Human SMG1 is one of the largest PIKK family members (~410 kDa) and plays a crucial role in nonsense-mediated mRNA decay (NMD), a conserved pathway that regulates mRNA stability in the cytoplasm of eukaryotic cells. In metazoans, SMG1 forms a stable complex with two additional proteins, SMG8 and SMG9, and specifically phosphorylates the RNA helicase UPF1. SMG1 phosphorylates UPF1 specifically at Ser/Thr - Gln (SQ) motifs present in the unstructured N- and C-terminal regions that flank the helicase core. Briefly, SMG1 consists of an N-terminal solenoid 'arch' and a compact C-terminal 'head' region.

For structure determination, we incubated SMG1-8-9 with UPF1-LSQ and AMPPNP, a non-hydrolyzable ATP analogue, and subjected the sample to cryo-EM single particle analysis. The final reconstruction reached an overall resolution of 2.9 Å (Figure 1—figure supplements 2 and 3), and allowed us to further complete and refine the published model for SMG1-8-9 (Gat et al., 2019). Importantly, compared to the previously published apo-SMG1-8-9 structure, the current reconstruction revealed extra density in the kinase active site accounting for both AMPPNP and UPF1-LSQ. The active site of SMG1 shows excellent density for residues 1075–1081 of UPF1-LSQ. The hydroxyl group of Ser1078, the phospho-acceptor residue in UPF1-LSQ, is positioned by residues of the catalytic loop, in particular Asp2335 and His2337. In our structure, the glutamine at position +1 of UPF1-LSQ reaches into a hydrophobic cage formed by the SMG1 activation segment and FATC domain. In particular, UPF1 Gln1079 stacks against Tyr3654 and Leu2365 and forms hydrogen bonds with the backbone of Val2367. In our model, the Leu residue at position −1 in the substrate forms a C-H⋅⋅⋅π-interaction with SMG1 Phe2215 and is further stabilized by hydrophobic interactions with SMG1 Pro2249 and Gly3656. The local resolution of around 3 Å allowed us to model SMG9-bound ATP in the reconstructed density, revealing the molecular basis for how the adenosine nucleotide is recognized by this unusual G-fold domain. In this manuscript, we report the first structure of a substrate-bound PIKK active site, thereby revealing the basis for phosphorylation site selection by SMG1 and other PIKK family members.

> XXXXXXXXXXXXXXXXXXXXXXXXXXXXXXXXXXXXXXXXXXXXXXXXXXXXXXXXXXXXXXXXXXXXXALETVGEKKAFSSVMQLVMTSLQSILENVDTPELLCKCVKCILLVARCYPHIFSTNFRDTVDILVGWHIDHTQKPSLTQQVSGWLQSLEPFWVADLAFSTTLLGQFLEDMEAYAEDLSHVASGESVDEDVPPPSVSLPKLAALLRVFSTVVRSIGERFSPIRGPPITEAYVTDVLYRVMRCVTAANQVFFSEAVLTAANECVGVLLGSLDPSMTIHCDMVITYGLDQLENCQTCGTDYIISVLNLLTLIVEQINTKLPSSFVEKLFIPSSKLLFLRYHKEKEVVAVAHAVYQAVLSLKNIPVLETAYKLILGEMTCALNNLLHSLQLPEACSEIKHEAFKNHVFNVDNAKFVVIFDLSALTTIGNAKNSLIGMWALSPTVFALLSKNLMIVHSDLAVHFPAIQYAVLYTLYSHCTRHDHFISSSLSSSSPSLFDGAVISTVTTATKKHFSIILNLLGILLKKDNLNQDTRKLLMTWALEAAVLMRKSETYAPLFSLPSFHKFCKGLLANTLVEDVNICLQACSSLHALSSSLPDDLLQRCVDVCRVQLVHSGTRIRQAFGKLLKSIPLDVVLSNNKHTEIQEISLALRSHMSKAPSNTFHPQDFSDVISFILYGNSHRTGKDNWLERLFYSCQRLDKRDQSTIPRNLLKTDAVLWQWAIWEAAQFTVLSKLRTPLGRAQDTFQTIEGIIRSLAAHTLNPDQDVSQWTTADNDEGHGNNQLRLVLLLQYLENLEKLMYNAYEGCANALTSPPKVIRTFFYTNRQTCQDWLTRIRLSIMRVGLLAGQPAVTVRHGFDLLTEMKTTSLSQGNELEVTIMMVVEALCELHCPEAIQGIAVWSSSIVGKNLLWINSVAQQAEGRFEKASVEYQEHLCAMTGVDCCISSFDKSVLTLANAGRNSASPKHSLNGESRKTVLSKPTDSSPEVINYLGNKACECYISIADWAAVQEWQNSIHDLKKSTSSTSLNLKADFNYIKSLSSFESGKFVECTEQLELLPGENINLLAGGSKEKIDMKKLLPNMLSPDPRELQKSIEVQLLRSSVCLATALNPIEQDQKWQSITENVVKYLKQTSRIAIGPLRLSTLTVSQSLPVLSTLQLYCSSALENTVSNRLSTEDCLIPLFSEALRSCKQHDVRPWMQALRYTMYQNQLLEKIKEQTVPIRSHLMELGLTAAKFARKRGNVSLATRLLAQCSEVQLGKTTTAQDLVQHFKKLSTQGQVDEKWGPELDIEKTKLLYTAGQSTHAMEMLSSCAISFCKSVKAEYAVAKSILTLAKWIQAEWKEISGQLKQVYRAQHQQNFTGLSTLSKNILTLIELPSVNTMEEEYPRIESESTVHIGVGEPDFILGQLYHLSSVQAPEVAKSWAALASWAYRWGRKVVDNASXXXXXXXXXXXXXXXXXXXXXXXXXXXXXXXXXXXXXXXXXXEGVIKVWRKVVDRIFSLYKLSCSAYFTFLKLNAGQIPLDEDDPRLHLSHRVEQSTDDMIVMATLRLLRLLVKHAGELRQYLEHGLETTPTAPWRGIIPQLFSRLNHPEVYVRQSICNLLCRVAQDSPHLILYPAIVGTISLSSESQASGNKFSTAIPTLLGNIQGEELLVSECEGGSPPASQDSNKDEPKSGLNEDQAMMQDCYSKIVDKLSSANPTMVLQVQMLVAELRRVTVLWDELWLGVLLQQHMYVLRRIQQLEDEVKRVQNNNTLRKEEKIAIMREKHTALMKPIVFALEHVRSITAAPAETPHEKWFQDNYGDAIENALEKLKXXXXXXXXXXXXXXXXYILRLEEISPWLAAMTNTEIALPGEVSARDTVTIHSVGGTITILPTKTKPKKLLFLGSDGKSYPYLFKGLEDLHLDERIMQFLSIVNTMFATINRQETPRFHARHYSVTPLGTRSGLIQWVDGATPLFGLYKRWQQREAALQAQKAQDSYQTPQNPGIVPRPSELYYSKIGPALKTVGLSLDVSRRDWPLHVMKAVLEELMEATPPNLLAKELWSSCTTPDEWWRVTQSYARSTAVMSMVGYIIGLGDRHLDNVLIDMTTGEVVHIDYNVCFEKGKSLRVPEKVPFRMTQNIETALGVTGVEGVFRLSCEQVLHIMRRGRETLLTLLEAFVYDPLVDWTAGGEAGFAGAVYGGGGQQAESKQSKREMEREITRSLFSSRVAEIKVNWFKNRDEMLVVLPKLDGSLDEYLSLQEQLTDVEKLQGKLLEEIEFLEGAEGVDHPSHTLQHRYSEHTQLQTQQRAVQEAIQVKLNEFEQWITHYQAAFNNLEATQLASLLQEISTQMDLGPPSYVPATAFLQNAGQAHLISQCEQLEGEVGALLQQRRSVLRGCLEQLHHYATVALQYPKAIFQKHRIEQWKTWMEELICNTTVERCQELYRKYEMQYAPQPPPTVCQFITATEMTLQRYAADINSRLIRQVERLKQEAVTVPVCEDQLKEIERCIKVFLHENGEEGSLSLASVIISALCTLTRRNLMMEGAASSAGEQLVDLTSRDGAWFLEELCSMSGNVTCLVQLLKQCHLVPQDLDIPNPMEASETVHLANGVYTSLQELNSNFRQIIFPEALRCLMKGEYTLESMLHELDGLIEQTTDGVPLQTLVESLQAYLRNAAMGLEEETHAHYIDVARLLHAQYGELIQPRNGSVDETPKMSAGQMLLVAFDGMFAQVETAFSLLVEKLNKMEIPIAWRKIDIIREARSTQVNFFDDDNHRQVLEEIFFLKRLQTIKEFFRLCGTFSKTLSGSSSLEDQNTVNGPVQIVNVKTLFRNSCFSEDQMAKPIKAFTADFVRQLLIGLPNQALGLTLCSFISALGVDIIAQVEAKDFGAESKVSVDDLCKKAVEHNIQIGKFSQLVMNRATVLASSYDTAWKKHDLVRRLETSISSCKTSLQRVQLHIAMFQWQHEDLLINRPQAMSVTPPPRSAILTSMKKKLHTLSQIETSIATVQEKLAALESSIEQRLKWAGGANPALAPVLQDFEATIAERRNLVLKESQRASQVTFLCSNIIHFESLRTRTAEALNLDAALFELIKRCQQMCSFASQFNSSVSELELRLLQRVDTGLEHPIGSSEWLLSAHKQLTQDMSTQRAIQTEKEQQIETVCETIQNLVDNIKTVLTGHNRQLGDVKHLLKAMAKDEEAALADGEDVPYENSVRQFLGEYKSWQDNIQTVLFTLVQAMGQVRSQEHVEMLQEITPTLKELKTQSQSIYNNLVSFASPLVTDATNECSSPTSSATYQPSFAAAVRSNTGQKTQPDVMSQNARKLIQKNLATSADTPPSTVPGTGKSVACSPKKAVRDPKTGKAVQERNSYAVSVWKRVKAKLEGRDVDPNRRMSVAEQVDYVIKEATNLDNLAQLYEGWTAWV;> MAGPVSLRDLLMGASAWMGSESPGGSPTEGGGSAAGGPEPPWREDEICVVGIFGKTALRLNSEKFSLVNTVCDRQVFPLFRHQDPGDPGPGIRTEAGAVGEAGGAEDPGAAAGGSVRGSGAVAEGNRTEAGSQDYSLLQAYYSQESKVLYLLLTSICDNSQLLRACRALQSGEAGGGLSLPHAEAHEFWKHQEKLQCLSLLYLFSVCHILLLVHPTCSFDITYDRVFRALDGLRQKVLPLLKTAIKDCPVGKDWKLNCRPCPPRLLFLFQLNGALKVEPPRNQDPAHPDKPKKHSPKRRLQHALEDQIYRIFRKSRVLTNQSINCLFTVPANQAFVYIVPGSQEEDPVGMLLDQLRSHCTVKDPESLLVPAPLSGPRRYQVMRQHSRQQLSFHIDSSSSSSSGQLVDFTLREFLWQHVELVLSKKGFDDSVGRNPQPSHFELPTYQKWISAASKLYEVAIDGKEEDLGSPTGELTSKILSSIKVLEGFLDIDTKFSENRCQKALPMAHSAYQSNLPHNYTMTVHKNQLAQALRVYSQHARGPAFHKYAMQLHEDCYKFWSNGHQLCEERSLTDQHCVHKFHSLPKSGEKPEADRNPPVLYHNSRARSTGACNCGRKQAPRDDPFDIKAANYDFYQLLEEKCCGKLDHINFPVFEPSTPDPAPAKNESSPAPPDSDADKLKEKEPQTQGESTSLSLALSLGQSTDSLGTYPADPQAGGDNPEVHGQVEVKTEKRPNFVDRQASTVEYLPGMLHSNCPKGLLPKFSSWSLVKLGPAKSYNFHTGLDQQGFIPGTNYLMPWDIVIRTRAEDEGDLDTNSWPAPNKAIPGKRSAVVMGRGRRRDDIARAFVGFEYEDSRGRRFMCSGPDKVMKVMGSGPKESALKALNSDMPLYILSSSQGRGLKPHYAQLMRLFVVVPDAPLQIILMPQVQPGPPPCPVFYPEKQEITLPPDGLWVLRFPYAYVTERGPCFPPKENVQLMSYKVLRGVLKAVTQ;> MSESGHSQPGLYGIERRRRWKEPGSGGPQNLSGPGGRERDYIAPWERERRDASEETSTSVMQKTPIILSKPPAERSKQPPPPTAPAAPPAPAPLEKPIVLMKPREEGKGPVAVTGASTPEGTAPPPPAAPAPPKGEKEGQRPTQPVYQIQNRGMGTAAPAAMDPVVGQAKLLPPERMKHSIKLVDDQMNWCDSAIEYLLDQTDVLVVGVLGLQGTGKSMVMSLLSANTPEEDQRTYVFRAQSAEMKERGGNQTSGIDFFITQERIVFLDTQPILSPSILDHLINNDRKLPPEYNLPHTYVEMQSLQIAAFLFTVCHVVIVVQDWFTDLSLYRFLQTAEMVKPSTPSPSHESSSSSGSDEGTEYYPHLVFLQNKARREDFCPRKLRQMHLMIDQLMAHSHLRYKGTLSMLQCNVFPGLPPDFLDSEVNLFLVPFMDSEAESENPPRAGPGSSPLFSLLPGYRGHPSFQSLVSKLRSQVMSMARPQLSHTILTEKNWFHYAARIWDGVRKSSALAEYSRLLA;> QPELSQDSYLG>[2x]I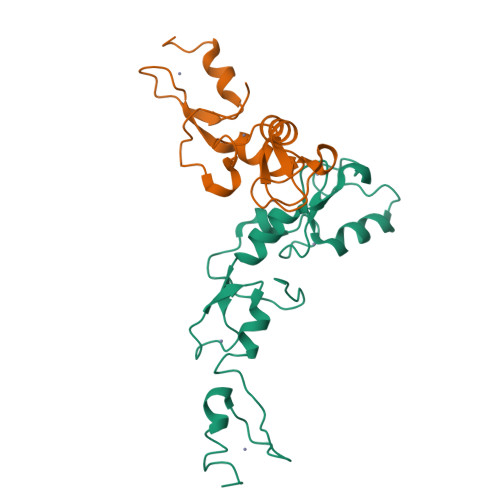SLDFEPSIEYQFVERLEERYKCAFCHSVLHNPHQTGCGHRFCQHCILSLRELNTVPICPVDKEVIKSQEVFKDNCCKREVLNLYVYCSNAPGCNAKVILGRYQDHLQQCLFQPVQCSNEKCREPVLRKDLKEHLSASCQFR;>[2x]EIQGYDVEFDPPLESKYECPICLMALREAVQTPCGHRFCKACIIKSIRDAGHKCPVDNEILLENQLFPDNFAKREILSLMVKCPNEGCLHKMELRHLEDHQAHCEFA>[2x]MSLNLKELFIHHLEKNLPKVESFHPFFNEALALMLKAGGKHFRAQLLLSVVQSNKPELLNQALDVALALEFIHTYSLIHDDLPAMDNADFRRGIPTLHKSYDETTAILVGDALNTEAFLVLSHAHLKDEIKIKLIKTLAFNAGLNGMVIGQAIDCFFEDKRLSLNELEFLHTHKTARLIAAALKMGCEICELNNEESNQIYKLGLKLGLIFQI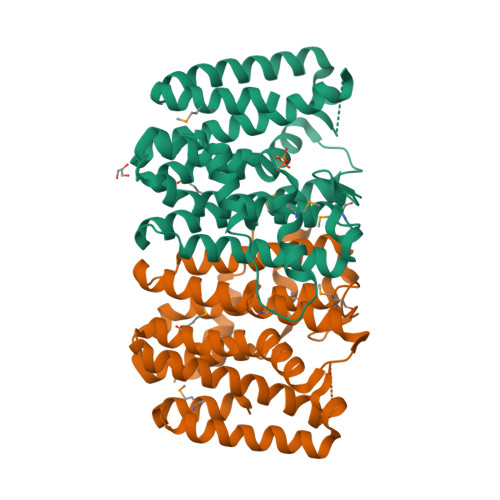NDDIIDVTTSQEQSGKPTNNDIHKNSFVNLLGLEQAIKTKENLLNECEQDLEKLNEKLAQMIQNLIIQYLEGHHHHHH3-(methylsulfanyl)benzoic acid | C8 H8 O2 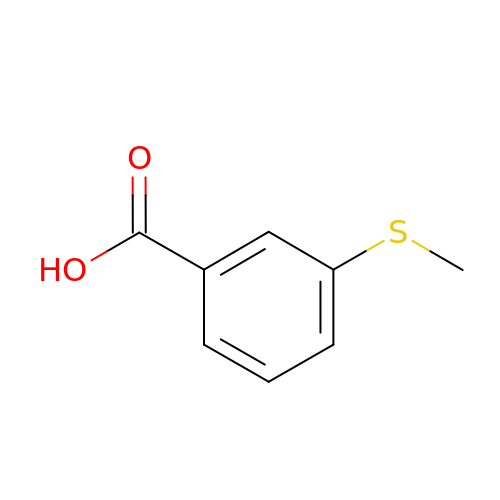S | PZGADOOBMVLBJE-UHFFFAOYSA-N>ERFKVVCYYTNWAWYRPDNGKYTPGDINPELCTHIIYAFAVLDKEELVIKSHDIWLDVENKFYEKVTALKSHGVKVLLGLGGWDDSAGDKYSRLVNNVSARRKFVVHAVDFLEQYGFDGLDLDWLYPKCWQVECEKGPDSDKQGFADLVKELRKAFNRRGMLLSAAVSASKRVIDYAYNVPALSMNLDWISLMTYDYHGQWDKKTGHVAPMYVHDKDTDNTFNVNFTVNYWINKGADRKKLVVGVPFYGQSFSVVEGAGTGLGAPTYAGGEAGDETRARGFLSFYEICERVKVKGWKVHRDPGGRIGPYATHDDQWVSFDDDFMARHKAEYVRAMELGGSMA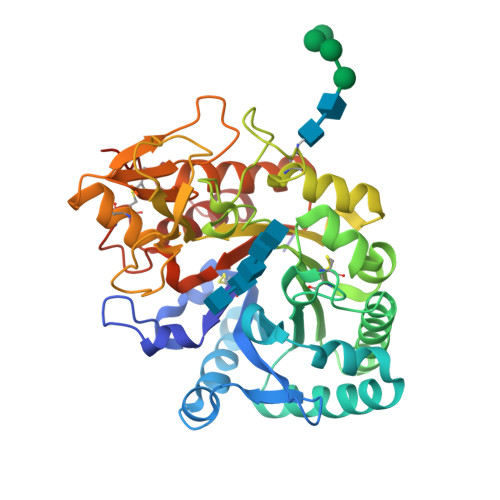WSLDLDDFTGKYCGCGKAPLLTTINHVLRGKEAPPPCILHE[2x]> MNFEGKIALVTGASRGIGRAIAETLAARGAKVIGTATSENGAQAISDYLGANGKGLMLNVTDPASIESVLEKIRAEFGEVDILVNNAGITRDNL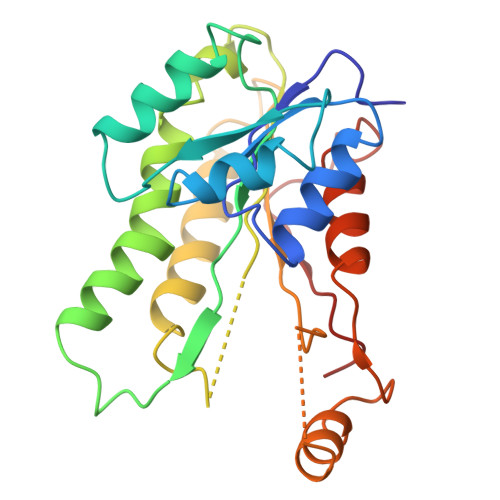LMRMKDEEWNDIIETNLSSVFRLSKAVMRAMMKKRHGRIITIGGQANYAAAKAGLIGFSKSLAREVASRGITVNVVAPGFIETSDDQRAGILAQVPAGRLGGAQEIANAVAFLASDEAAYITGETLHVNGGM> SRIVDPKFSSPIVNMTAPVGRDAFLTCVVQD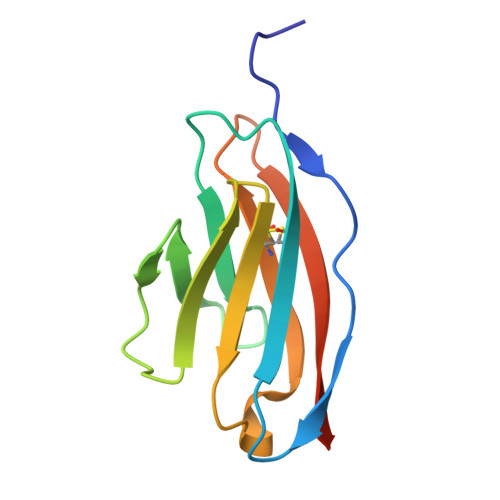LGPYKVAWLRVDTQTILTIQNHVITKNQRIGIANSEHKTWTMRIKDIKESDKGWYMCQINTDPMKSQMGYLDVVVHHHHHH> GPVPMHPFVKALQEHFTAHQNPEKAEPMARYMKNHFLFLGIQTPERRQLLKDIIQIHTLPDQKDFQIIIRELWDLPEREFQAAALDIMQKYKKHINETHIPFLEELIVTKSWWDSVDSIVPTFLGDIFLKHPELISAYIPKWIASDNIWLQRAAILFQLKYKQK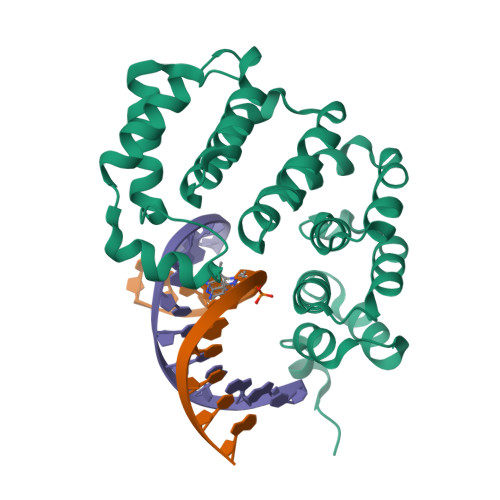MDEELLFWIIGQLHSSKEFFIQKAIGWVLREYAKTNPDVVWEYVQNNELAPLSKREAIKHIKQNYGINN> EFRHDSRKIPKVGHTFFQKPESCPPVPGGSMKLDIGIINENQRVSMSRNIESRSTSPWNYTVTWDPNRYPSEVVQAQCRNLGCINAQGKEDISMNSVPIQQETLVVRRKHQGCSVSFQLEKVLVTVGCTCVTPVIHHVQ;> LERLVGPQDATHCSPGLSCRLWDSDILCLPGDIVPAPGPVLAPTHLQTELVLRCQKETDCDLCLRVAVHLAVHGHWEEPEDEEKFGGAADSGVEEPRNASLQAQVVLSFQAYPTARCVLLEVQVPAALVQFGQSVGSVVYDCFEAALGSEVRIWSYTQPRYEKELQHTQQLPDCRGLEVWNSIPSCWALPWLNVSADGDNVHLVLQVSEEQHFGLSLYWNQVQGPPKPRWHKQLTGPQIITLQHTDLVPCLCIQVWPLEPDSVRT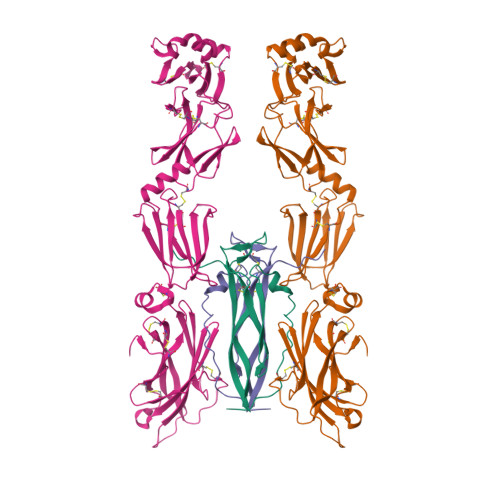NICPFREDPRAHQNLWQAARLRLLTLQSWLLDAPCSLPAEAALCWRAPGGDPCQPLVPPLSWEQVTVDKVLEFPLLKGHPNLCVQVQSSEKLQLQECLWADSLGPLKDDVLLLETRGPQDQRSLCALEPSGCTSLPSKASTRAARLGEYLLQDLQSGQCLQLWDDDLGALWACPMDKYIHKREFRH>[3x]FSNLAIYWGQGPNQLRLSHFCQETSLDIINI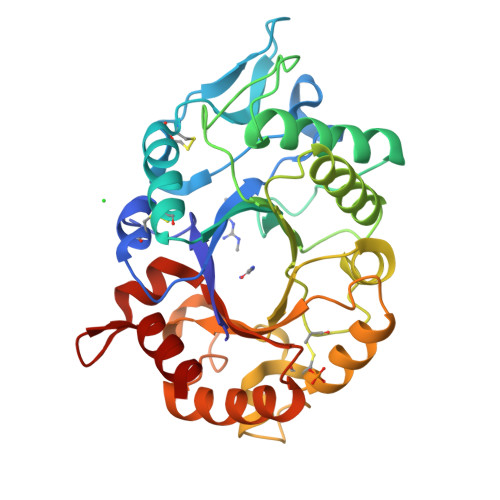GFINYFPDMSPGHWPGSNFGNQCDGSVYVTNDGVVTKLLSGCHQIMEDIPICQAAGKKVLLSIGGAYPPDQSILSEDSAVAFATFLWGAFGPVAEGWEGPRPFGDVVVDGFDFDIEHNGGFGYATMVNTFRQYFNQVPERKFYLSAAPQCIIPDAQLSDAIFNAAFDFIWIQYYNTAACSAKSFIDTSLGTFNFDAWVTVLKASASKDAKLYVGLPASETAANQGYYLTPDEVESLVSTYMDRYPDTFGGIMLWEATASENNQIDGAPYADHMKDILLH6-{[(CYCLOHEXYLAMINO)CARBONYL]AMINO}HEXANOIC ACID | C13 H24 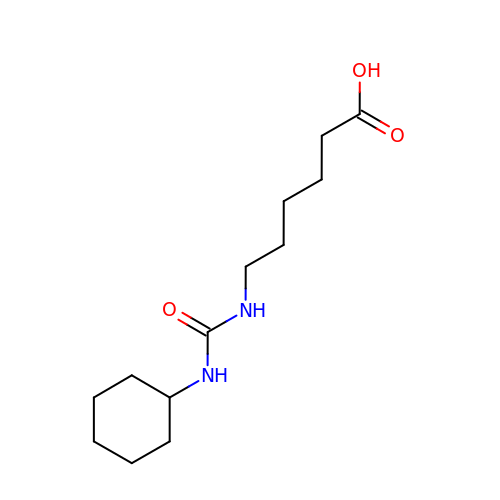N2 O3 | KFTVEPYSUSWBRD-UHFFFAOYSA-N> MDFNLSNSQSDIYESAYRFACDVLDQDAQTRISQKILSTELWKKAAAYGFAHGPVSHQFGGSELGALDTALMIEALGKGSRDIGLSFSLCAHLCACVIPLYRFGSSELKDKYLESLVTGKLIAANAATEPDAGSDIYNMQATAQPCEGGYILNGKKIFITNAPIADVFIIYAKTNPDHGFLGVSAFLIEKGTPGLNVGEVIPKDCLSNCPWSEIVFNDIFIPQSQRIGMEGAGGAIFHD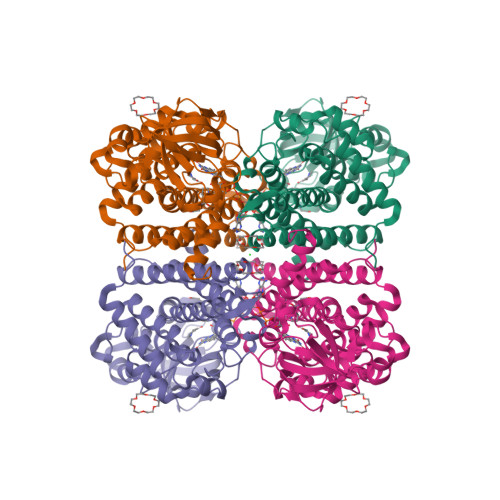SMIWAKGCLSALFVGGLARLLETTLEYAKARQQFGKAIGQFQSVSNRIIDMKLRLEQCRLMLYRACWKHDQGQDAEADIAMSKLLISEYAVQSGLDAIQTFGGAAMDQELGLVRHLLNMIPSRIFSGTNDIQKEIIARKLGLRGTSSGSLVPRGSHHHHHHHH> GPLGSNRKRLPSYLKPGSAVEISSDEIGFRGSWYMGKVITIPSSSDKDSVKCQVEYTTLFFDKEGTKPLKEVVDMSQLRPPAPPMSEIEKKKKIVVGEEVDAFYNDGWWEGDVTEVLDDGKFSVFFRSSKEQIRFRKDELRFHR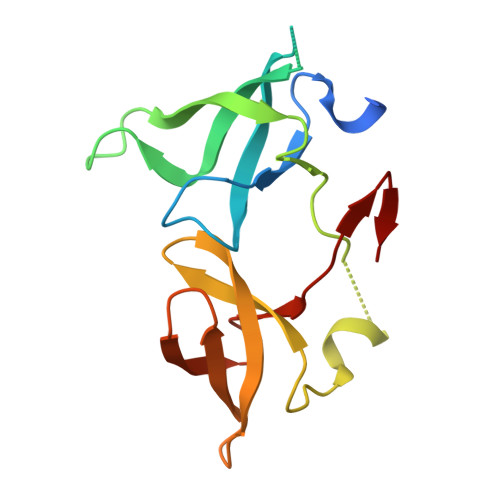EWVDGAWK> MFERFTDRARRVVVLAQEEARMLNHNYIGTEHILLGLIHEGEGVAAKSLESLGISLEGVRSQVEEIIGQGQQAPSGHIPFTPRAKKVLELSLREALQLGHNYIGTEHILLGLIREGEGVAAQVLVKLGAELTRVRQQVIQLLSGYKLAAALEHHHHHH

ClpC1 is an ATP-dependent homohexamer that is responsible for substrate recognition and unfolding. ClpC1 is a 95 kDa caseinolytic AAA+ protein with an N-terminal domain (NTD) and two nucleotide-binding domains (D1 and D2). The essential ClpC1–ClpP1–ClpP2 proteasome complex of Mtb has recently become the focus of several drug-discovery campaigns. The NTD (amino acids 1–145) has been studied extensively to determine the most critical residues for the binding of ClpC1 to several natural cyclopeptides with potent anti-TB activity.

Excluding the four N-terminal residues, the r.m.s.d.s between these two apo structures and that with bound ECU (chain W) are 0.43 and 0.68 Å, respectively, explaining the importance of these structures in solving the large asymmetric unit of the ClpC1-NTD–ECU complex. In addition, the N-terminus of ClpC1-NTD maintains a distinct 310-helical structure in the RUF-I and CYMA complexes, rigidified by the covalent bond with Met1, while the N-terminus is more extended in the apo structures and in the ECU complex. In addition, helices 4–5 and 8–9 were shifted by about 3–4 Å owing to a pivot point in the 70s loop. It was observed that one conformation is captured in the apo form and the RUF-I and CYMA complexes, with a second conformation being captured when ECU was bound, in solution or in the ECU-resistant double mutant ClpC1-NTD-L92S/L96P. Apart from the protein termini, the 70s loop is the most flexible portion of the NTD structures. The region consistently has higher B factors and was more challenging to refine, with unusual orientations of residues. This may reflect the true nature of the protein itself; the mobility of this loop may allow the domain movements that are observed between structures.> MGSSHHHHHHSQDPNSMTTLTRQDLN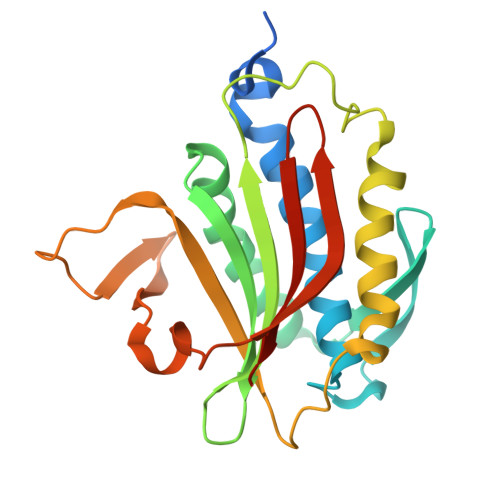FGQVVADVLCEFLEVAVHLILYVREVYPVGIFQARKKYNVPVQMSCHPELNQYIQDTLHCVKPLLEKNDVEKVVVVILDKEHRPVEKFVFEITQPPLLSISSDSLLSHVEQLLAAFILKISVCDDVLDHNPPGCTFTVLVHTREAATRNMEKIQVIKDFPWILADEQDVHMHDPRLIPLKTMTSDILKMQLYVEERAHKGS BETA(2-THIENYL)ALANINE | C7 H9 N O2 S | 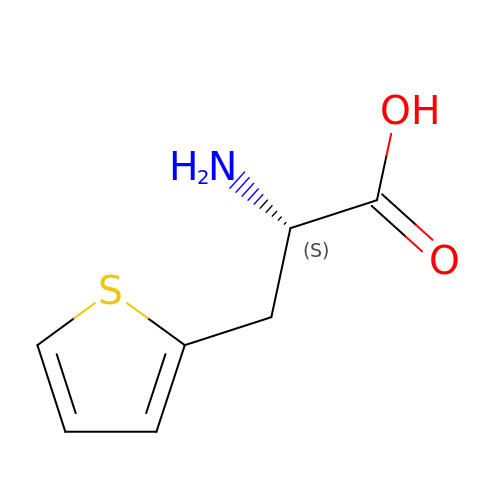WTOFYLAWDLQMBZ-LURJTMIESA-N> MCPPGWSSNGVYCYMLFKEPKTWDEAEKFCNKQGKDGHLLSIESKKEEILVDIVVSENIGKMYKIWTGLSERSKEQHCSSRWSDGSFFRSYEIAIRYSECFVLEKQSVFRTWVATPCENTFPFM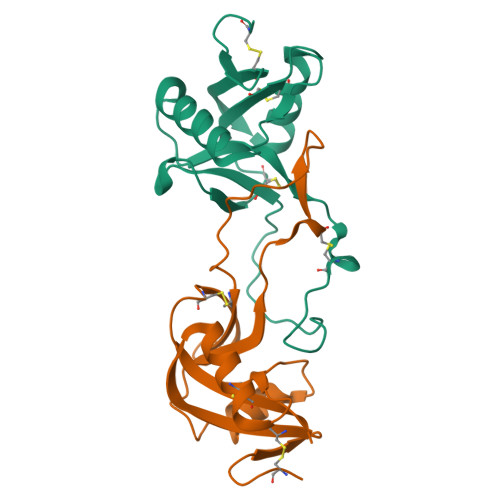CKYPVPR;> NCLPDWSVYEGYCYKVFKERMNWADAEKFCTKQHKDGHLVSFRNSKEVDFVISLAFPMLKNDLVWIGLTDYWRDCNWEWSDGAQLDYKAWDNERHCFIYKNTDNQWTRRDCTWTFSFVCKCPA>[2x]MAHHHHHHMSERVILAYSGGLDTSVAISWIGKETGREVVAVAIDLGQGGEDMEVVRQRALDCGAVESIVIDARDEFANDYCVPAIQSNALYMDRYPLVSALSRPLIVKHLVKAAREHGGTIVAHGCTGKGN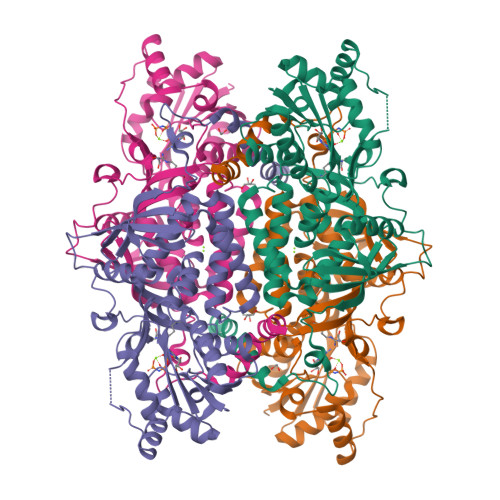DQVRFEVGFASLAPDLEVLAPVRDYAWTREKAIAFAEENNIPINVTKRSPFSIDQNVWGRAVETGFLEHLWNAPTKDVYSYTEDPTVNWSTPDEVIVGFEQGVPVSIDGRSVTPLQAIEELNRRGGEQGVGRLDVVEDRLVGIKSREIYEAPGAMVLITAHTELEHVTLERELGRFKRITDQKWGELVYDGLWFSPLKTALESFVAKTQEHVTGEIRMVLHGGHIAVNGRRSPKSLYDFNLATYDEGDTFDQSAAKGFVQIHGLSSSISARRDLQGQ> MSTIKPVSVKLDADIKARVEHLAETRKRSSHWMMREAIREYVEREEKREALQQEALRA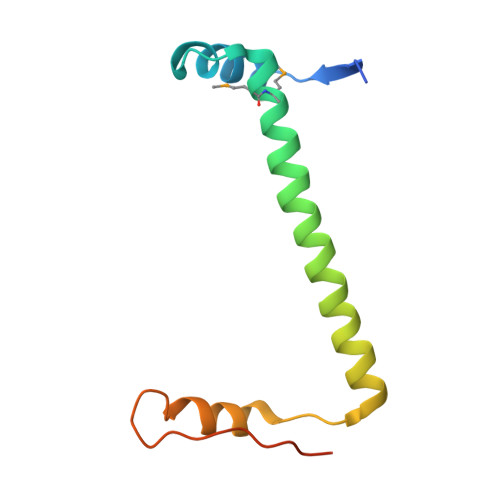WEEHQTSGLHVTGDEVVSWLESWGSENEQAALHATNSLHCHCIT> METREHLFKVLV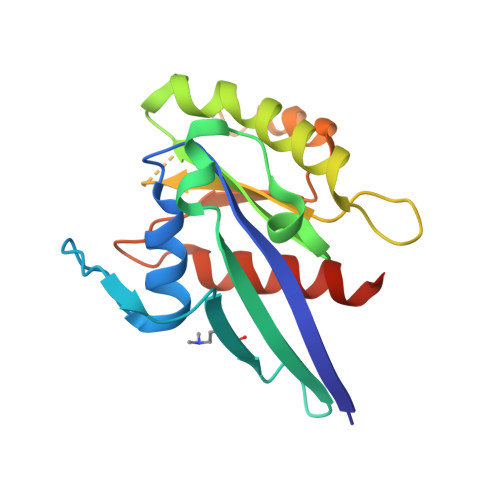IGELGVGKTSIIKRYVHQLFSQHYRATIGVDFALKVLNWDSRTLVRLQLWDIAGQERFGNMTRVYYKEAVGAFVVFDISRSSTFEAVLKWKSDLDSKVHLPNGSPIPAVLLANKCDQNKDSSQSPSQVDQFCKEHGFAGWFETSAKDNINIEEAARFLVEKILVNHQSFPN> R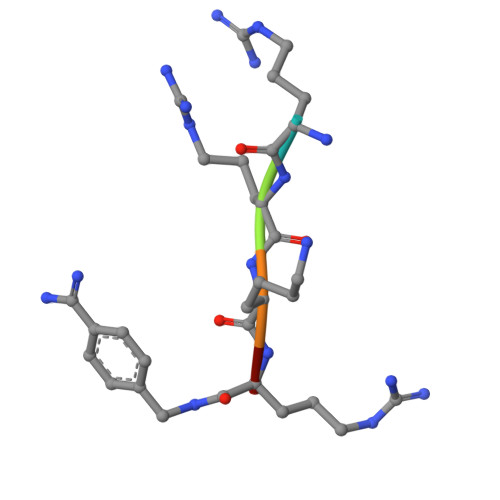RKRX>XRITRLQEKEDLQELNDRLAVYIDRVRSLETEN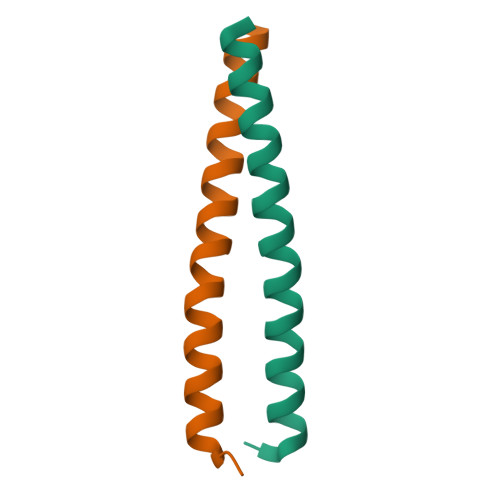AGLRLRITEX[4x]> GLEDCDFGWSPYDQHCYQAFNEQKTWDEAEKFCRAQENGAHLASIESNGEADFVSWLISQKDELADEDYVWIGLRAQNKEQQCSSEWSDGSSVSYENLIDLHTKKCGAL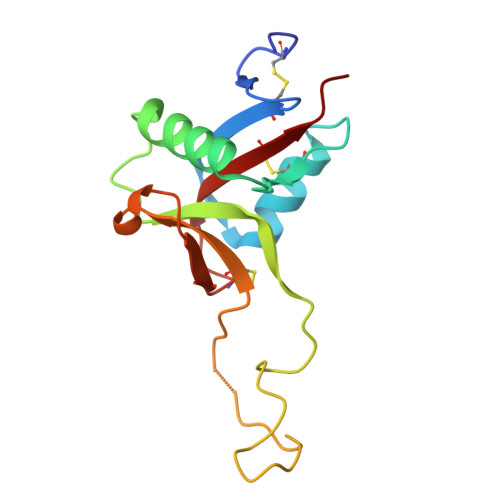EKLTGFRKWVNYYCEQMHAFVCKLLPY>MKKGHHHHHHTSCNPSDMSHGYVTVKPRVRLHFVELGSGPAVCLCHGFPESWYSWRYQ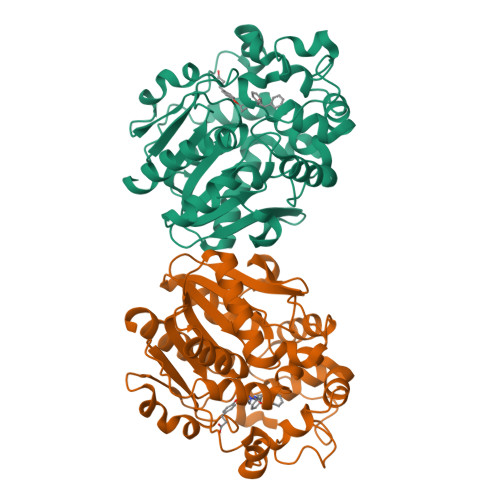IPALAQAGYRVLAMDMKGYGESSAPPEIEEYCMEVLCKEMVTFLDKLGLSQAVFIGHDWGGMLVWYMALFYPERVRAVASLNTPFIPANPNMSPLESIKANPVFDYQLYFQEPGVAEAELEQNLSRTFKSLFRASDESVLSMHKVCEAGGLFVNSPEEPSLSRMVTEEEIQFYVQQFKKSGFRGPLNWYRNMERNWKWACKSLGRKILIPALMVTAEKDFVLVPQMSQHMEDWIPHLKRGHIEDCGHWTQMDKPTEVNQILIKWLDSDARNPPVVSKM[2x]> AYTTFSQTKNDQLKEPMFFGQPVNVARYDQQKYDIFEKLIEKQLSFFW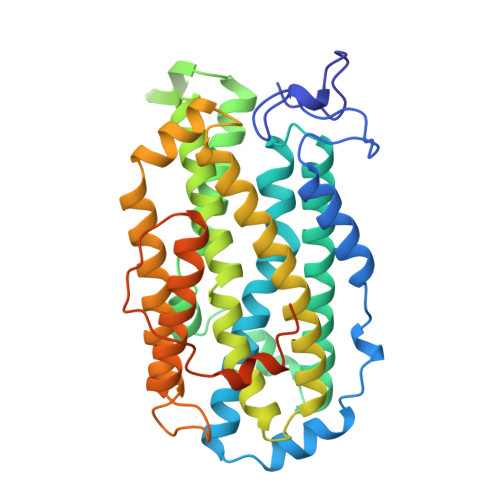RPEEVDVSRDRIDYQALPEHEKHIFISNLKYQTLLDSIQGRSPNVALLPLISIPELETWVETWAFSETIHSRSFTHIIRNIVNDPSVVFDDIVTNEQIQKRAEGISSYYDELIEMTSYWHLLGEGTHTVNGKTVTVSLRELKKKLYLCLMSVNALEAIRFYVSFACSFAFAERELMEGNAKIIRLIARDAALHLTGTQHMLNLLRSGADDPEMAEIAEECKQECYDLFVQAAQQEKDWADYLFRDGSMIGLNKDILCQYVEYITNIRMQAVGLDLPFQTRSNPIPWINTWLVSDNVQVAPQEVEVSSYLVGQIDSEVDTDDLSNFQL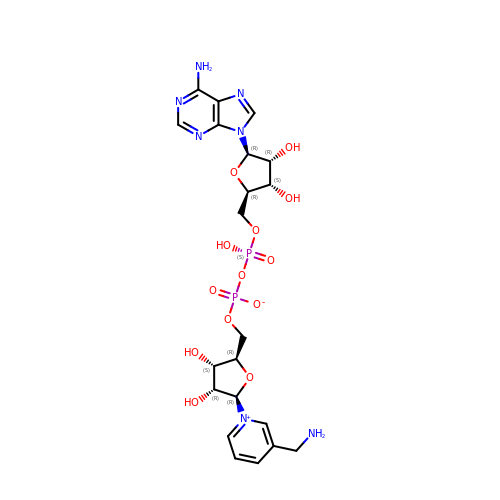3-AMINOMETHYL-PYRIDINIUM-ADENINE-DINUCLEOTIDE | C21 H29 N7 O13 P2 | HMCRLFVYYFBZEZ-PLEFRAQWSA-N3,3'-(3,7,12,17-tetramethylporphyrin-2,18-diyl)dipropanoic acid | C30 H30 N4 O4 | 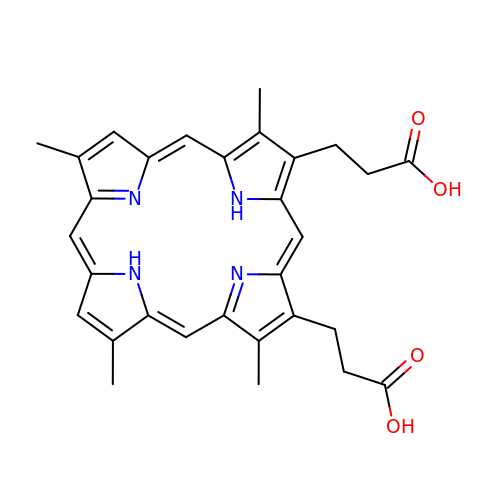VVNYLNWIIBXFLK-LMKUSPAJSA-N> METITVSTPIKQIFPDDAFAETIKANLKKKSVTDAVTQNELNS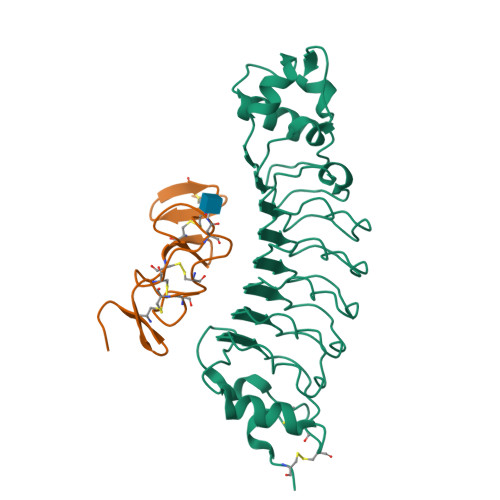IDLISAPHSDIKSVQGIQYLPNVRLLYLGGNKLHDISALKELTNLTTLILSGNQLQSLPNGVFDKLTNLKVLWLSVNQLQSLPDGVFDKLTNLTSLRLHRNQLQSLPKGVFDKLTNLTVLRLSENQLQSLPEGVFDKLTQLKVLWLGRNQLKSVPDGVFDRLTSLQYIWLHDNPWDCTCPGIRYLSEWINKHSGVVRNSAGSVAPDSAKCSGSGKPVRSIICPTLEHHHHHH;> QCSQFLRGQECVEECRVLQGLPREYVNARHCLPCHPECQPQNGSVTCFGPEADQCVACAHYKDPPFCVARCPSGVKPDLSYMPIWKFPDEEGACQPC>[2x]MSKIDFHTHYLPTSYVEALKRHVPGDPDGWPTPEWTPQLTLNFMRDNDISYSILSLSSPHVNFGDKAETIRLVEAANDDGKSLAQ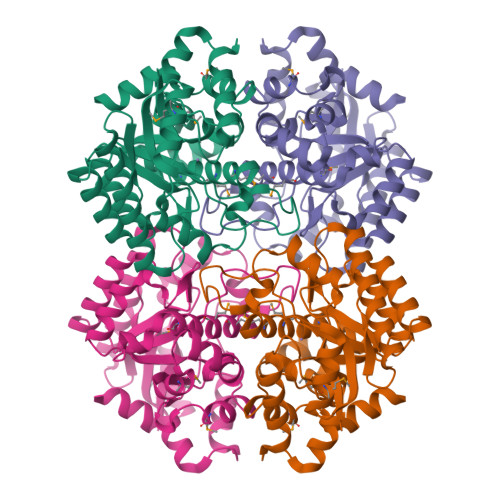QYPDQLGYLASLPIPYELDAVKTVQQALDQDGALGVTVPTNSRGLYFGSPVLERVYQELDARQAIVALHPNEPAILPKNVDIDLPVPLLGFFMDTTMTFINMLKYHFFEKYPNIKVIIPHAGAFLGIVDDRIAQYAQKVYQVDVYDVMHHVYFDVAGAVLPRQLPTLMSLAQPEHLLYGSDIPYTPLDGSRQLGHALATTDLLTNEQKQAIFYDNAHRLLTE>[2x]GPSSSKSEENISLVYEIDGTE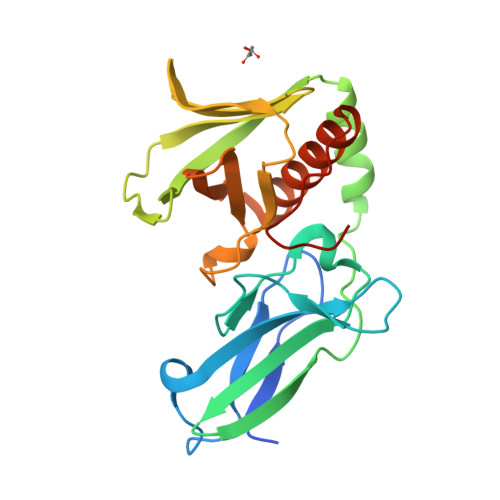ALGSCLRVRPCSNDAPDLSKCTIQWYRSSSDGSKKELISGATKSVYAPEPFDVGRVLHADIIYDGHSLSLSTVGKIDPAAGLGSYVEALVRKHDVDFNVVVTQMSGEDHTSESIHLFHVGKMRIKLCKGKTVIAKEYYSSAMQLCGVRGGGNAAAQALYWQAKKGVSFVIAFESERERNAAIMLARRFACDCNVTLAGPEDRTETGQSP> GSGGSHMGSGRIELNSVSFRYNGDYVLKDVNAEFETGKIYVVVGKNGSGKTTLLKILAGLLAAAGEIFLD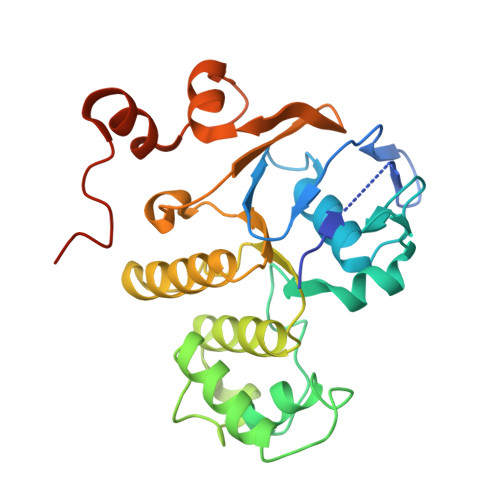GSPADPFLLRKNVGYVFQNPSSQIIGATVEEDVAFSLEIMGLDESEMRKRIKKVLELVGLSGLAAADPLNLSGGQKQRLAIASMLARDTRFLALDEPVSMLDPPSQREIFQVLESLKNEGKGIILVTHELEYLDDMDFILHISNGTIDFCGSWEEFVEREFDDVEIPFKWKLWKKCGKINLWEDRYENSGNQRRRDTV> SDLLAWDPLF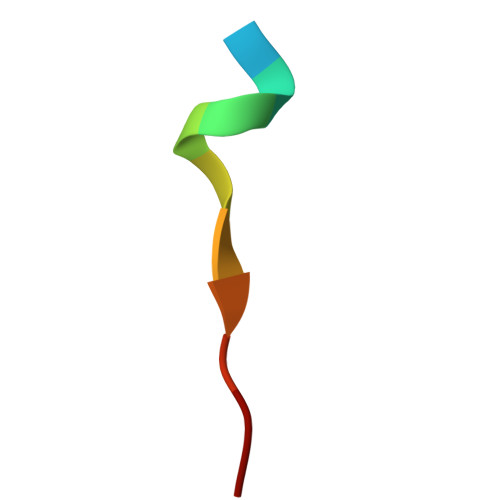G Canonically, CDKs require cyclin binding and phosphorylation of the kinase activation segment (T-loop) for full catalytic activity. Aberrant CDK4/6 activity and dysregulation of this signaling axis is frequent in multiple cancer types and it has emerged as an actionable drug target. Of particular interest, phosphorylation of CDK4 at T172 (pT172) is critical for generating the active conformation, yet no such crystal structure has been reported to date. However, the protein structures of CDK4 reported to date exhibit a conformation incompatible with catalysis and binding of ATP or ATP-competitive inhibitors.

Here, we determine the first x-ray crystal structure of active CDK4 in complex with cyclin D3, in the presence of the CDK4/6 inhibitor abemaciclib. We determined the structure by molecular replacement with a model of active CDK623 and cyclin D313. The final refined model displayed the canonical features of an active CDK including an “in” αC-helix, ordered activation segment and unambiguous electron density at Threonine 172 that indicated phosphorylation (pT172), a state required for maximal CDK4 activity. In contrast with the kinase domain, minimal structural changes to cyclin D3 were evident, except for the N-terminus, which becomes largely ordered (residues 11–22), and extensively interacts with the CDK4 activation segment. C The cyclin D3 N-terminus (ordered after residue H11) buttresses the activation segment, playing a role in adoption of the active conformation. Residues R14 and E74 form an “electrostatic belt” around the activation segment.

> XATSRYEPVAEIGVGAYGTVYKARDPHSGHFVALKSVRVPNGGGGGGGLPISTVREVALLRRLEAFEHPNVVRLMDVCATSRTDREIKVTLVFEHVDQDLRTYLDKAPPPGLPAETIKDLMRQFLRGLDFLHANCIVHRDLKPENILVTSGGTVKLADFGLARIYSYQMALTPVVVTLWYRAPEVLLQSTYATPVDMWSVGCIFAEMFRRKPLFCGNSEADQLGKIFDLIGLPPEDDWPRDVSLPRGAFPPRGPRPVQSVVPEMEESGAQLLLEMLTFNPHKRISAFRALQHSYLHKDEGNPEEGHHHHHH;> MELLCCEGTRHAPRAGPDPRLLGDQRVLQSLLRLEERYVPRASYFQCVQREIKPHMRKMLAYWMLEVCEEQRCEEEVFPLAMNYLDRYLSCVPTRKAQLQLLGAVCMLLASKLRETTPLTIEKLCIYTDHAVSPRQLRDWEVLVLGKLKWDLAAVIAHDFLAFILHRLSLPRDRQALVKKHAQTFLALCATDYTFAMYPPSMIATGSIGAAVQGLGACSMSGDELTELLAGITGTEVDCLRACQEQIEAALRESLREAS> LPTSNPAQELEARQLERTTRDDLINGNSASCADVIFIYARGSTETGNLGTLGPSIASNLESAFGKDGVWIQGVGGAYRATLGDNALPRGTSSAAIREMLGLFQQANTKCPDATLIAGGYSQGAALAAASIEDLDSAIRDKIAG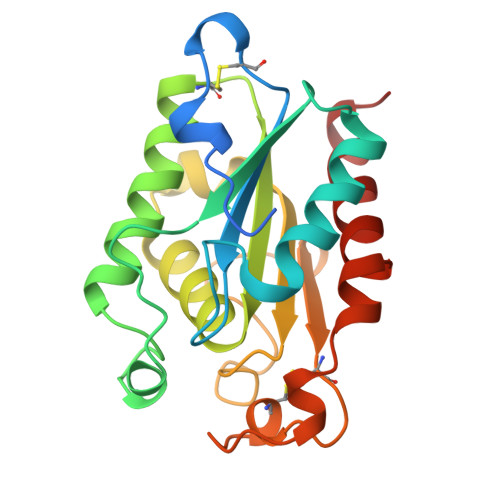CVLFGYTKNLQNRGRIPNYPADRTKVFCNTGDLVCTGSLIVAAPHLAYGPDARGPAPEFLIEKVRAVRGSA> MPKALRFLGWPVLVGVLLALLIIQHNPELVGLPRQEVHVEQAPLLSRLQEGPVSYANAVSRAAPAVANLYTTKMVSKPSHPLFDDPMFRRFFGDNLPQQKRMESSLGSAVIMSAEGYLLTNNHVTAGADQIIVALRDGRETIAQLVGSDPETDLAVLKIDLKNLPAMTLGRSDGIRTGDVCLAIGNPFGVGQTVTMGIISATGRNQLGLNTYEDFIQTDAAINPGNAGGALVDAAGNLIGINTAIFSKSGGSQGIGFAIPTKLALEVMQSIIEHGQVIRGWLGVEVKALTPELAESLGLGETAGIVVAGVYRDGPAARGGLLPGDVILTIDKQEASDGRRSMNQVARTRPGQKISIVVLRNGQKVNLTAEVGLRPPPAPAPQQKQDGGE;> WVF

AlgW, a membrane-bound periplasmic serine protease belonging to the HtrA protein family, is a key regulator of the regulated intramembrane proteolysis (RIP) pathway and is responsible for transmitting the envelope stress signals in Pseudomonas aeruginosa. The AlgW PDZ domain senses and binds the C-terminal of mis-localized outer membrane proteins (OMPs) or periplasmic protein MucE, leading to catalytic activation of the protease domain. HtrA protease is characterized by its trypsin-like catalytic domain and regulatory PDZ domain; the catalytic triad was surrounded by several loops (L1, L2, L3, LD, LA) but, usually, in an inactive mode, and could be activated by sensing a specific molecular stimulus. The catalytic triad (H123, D153, and S227) sites are located between two β-barrels and are surrounded by activation loops L1 to L3, LD, and LA (named according to DegS nomenclature).

In order to elucidate the structural basis of the AlgW reaction mechanism, we prepared the periplasmic soluble domain of AlgW and its inactive mutant AlgWS227A. Protein samples were mixed with two types of peptide activator (tripeptide WVF, decapeptide SVRDELRWVF) prior to crystallization trials, yielding four complex structures, AlgW-tripeptide, AlgWS227A-tripeptide, AlgW-decapeptide, and AlgWS227A-decapeptide, with resolutions from 1.8 to 2.6 Å. AlgW-tripeptide and AlgWS227A-tripeptide crystals belong to the P6322 space group. They have only one complex in an asymmetric unit, and their overall structures are similar (the root mean square deviation [RMSD] value was 1.07 Å). The AlgW trimer could be generated by symmetry operation, and similar to most HtrA protease, this funnel-like trimeric organization is mainly mediated by the N-terminal protease domains. Because of the high flexibility, our AlgW-tripeptide and AlgWS227A-tripeptide structures, as well as many HtrA protease structures, lack the LA loops. Consistently, AlgW-peptide bound structures also demonstrated different interdomain orientations, in which the joint angles of the PDZ relative to the protease domain are AlgW-WVF (25.62°) < AlgWS227A-WVF (25.74°) < AlgW-decapeptide (25.47 to 26.48°; average, 26.13°) < AlgWS227A-decapeptide (26.65°). Thus, by recognizing additional C-terminal residues of the targeting protein, the PDZ domain of AlgW adopts a more open form and maintains a more stable state, generating stronger substrate cleavage activity. This is in accordance with our enzymatic assay in which the tripeptide-bound AlgW is partially activated, while the decapeptide-bound structures reflect the further activation of AlgW.>AAPSFDCGKPQVEPKKCPGRVVGGCVAHPHSWPWQVSLRTRFGMHFCGGTLISPEWVLTAAHCLEKSPRPSSYKVILGAHQEVNLEPHVQEIEVSRLFLEPTRKDIALLKLSSPAVITDKVIPACLPSPNYVVADRTECFITGWGETQGTFGAGLLKEAQLPVIENKVCNRYEF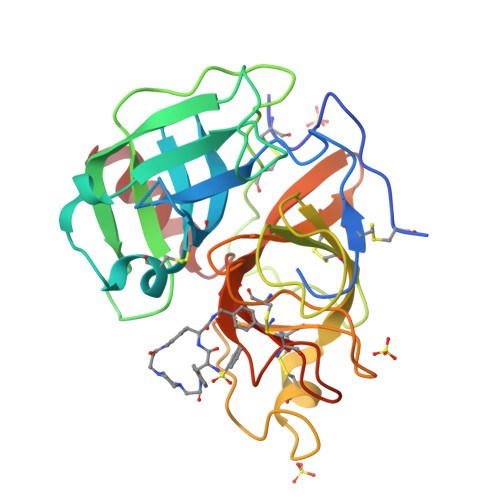LNGRVQSTELCAGHLAGGTDSCQGDAGGPLVCFEKDKYILQGVTSWGLGCARPNKPGVYVRVSRFVTWIEGVMRNN[2x]N-(4-fluorobenzoyl)-L-gamma-glutamyl-5-{[(S)-{[(1S)-1,3-dicarboxypropyl]amino}(hydroxy)phosphoryl]oxy}-L-norvaline 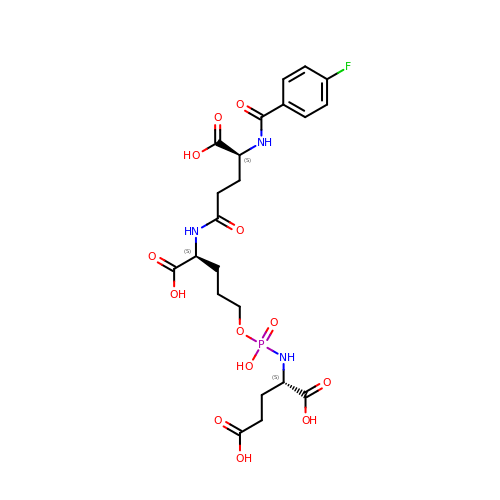| C22 H29 F N3 O13 P | RHOKGKWGPOEIFI-JYJNAYRXSA-N>SGTVTFDITNIDWETAEWIMKHVYLIAKKEGTDVTFSFKEGELQITVKNLHEEAKREIEKWIRAAQLAQDPDAESKAEARKILNELITEKAEELREKTKDEEVRELAREAARLALESDDIEVQRVVLKALLAALKSKDEEVIRLLLLAAVLAAAAARSGSPEEKLEIAKKALELAMKSKDEEVIRLALLAAVLAARSDDEEVLKKVKEALEKMERIMDLEDVAREKSGSAEASQAVKEIADIAEEALREGLCEVARVALKRLFKLAKDYPGSDVASLAKKALEKIAETALRNGCKETAEL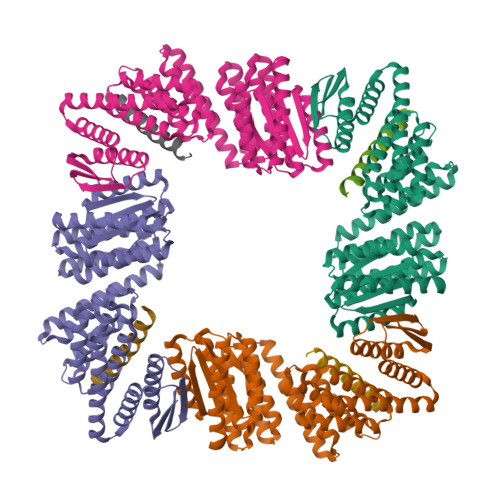AKLLLFLLLIIEVVLKMGVRMLTHRGGNAVIVVIEGLHPSQIVQLMQDVIKAAKKLGVTVTITVSGDIVVIMVVVGASDEEQEEARRLVQEIARALQEAKRKGANEEQLEQLLRELLERAEREGGSG[4x];>EERKKELAKEVIETAKKLIEKLAKEE[4x]>MFGLIGHLTSLEQARDVSRRMGYDEYADQGLEFWSSAPPQIVDEITVTSATGKVIHGRYIESCFLPEMLAARR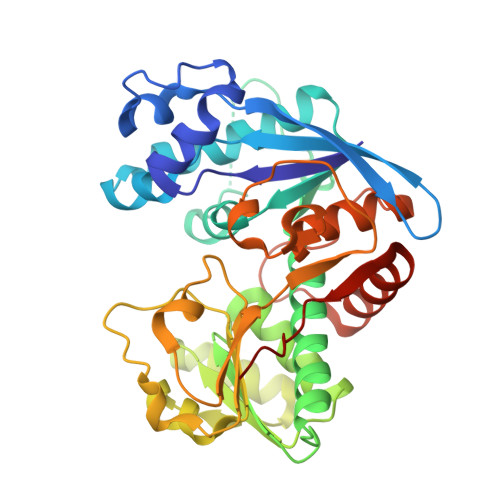FKTATRKVLNAMSHAQKHGIDISALGGFTSIIFENFDLASLRQVRDTTLEFERFTTGNTHTAYVICRQVEAAAKTLGIDITQATVAVVGATGDIGSAVCRWLDLKLGVGDLILTARNQERLDNLQAELGRGKILPLEAALPEADFIVWVASMPQGVVIDPATLKQPCVLIDGGYPKNLGSKVQGEGIYVLNGGVVEHCFDIDWQIMSAAEMARPERQMFACFAEAMLLEFEGWHTNFSWGRNQITIEKMEAIGEASVRHGFQPLALAIENLYFQ[5x]> GMDTQQLYFLNDIGKQKPESIRNRSAACPFCDRENLTD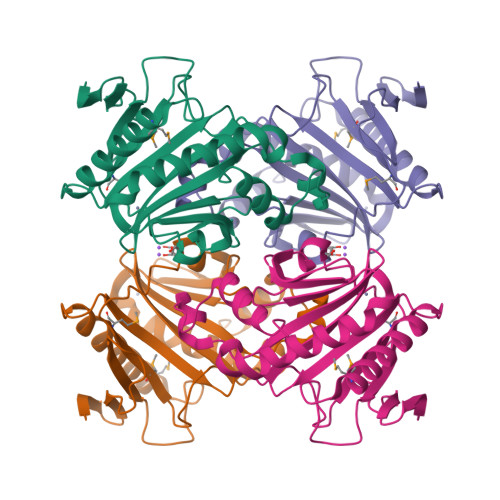ILATEGSIIWLKNKFPTLKDTFQTVLIETDNCEDHIATYTEEHMRSLIRFSIKHWLNLQKNEEFTSVILYKNHGPFSGGSLHHAHMQIIGMKYVNYLDNVEQDNFQGVIVQKNEHIELNISDRPIIGFTEFNIIIEDIGCIDELANYIQQTVRYILTDFHKGCSSYNLFFYYLNEKIICKVVPRFVVSPLYVGYKIPQVSTKIEDVKIQLAAYFTKQNDAIIHKKIE> QSSVTLFGIVDTNVAYVNKDAAGDSRYGLGTSGASTSRLGLRGTEDLGGGLKAGFWLEGEIFGDDGNASGFNFKRRSTVSLSGNFGEVRLGRDLVPTSQKLTSYDLFSATGIGPFMGFRNWAAGQGADDNGIRANNLISYYTPNFGGFNAGFGYAFDEKQTIGTADSVGRYIGGYVAYDNGPLSASLGLAQQKTAVGGLATDRDEITLGASYN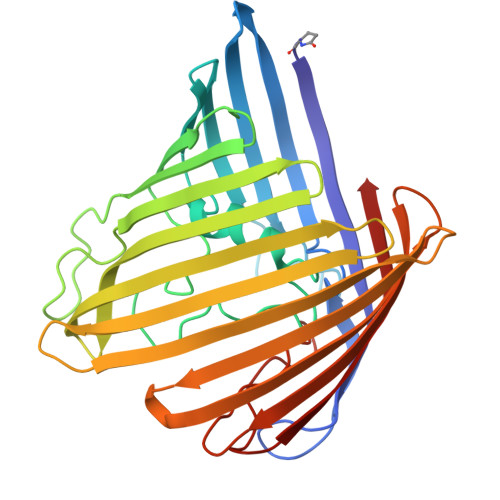FGVAKLSGLLQQTKFKRDIGGDIKTNSYMLGASAPVGGVGEVKLQYALYDQKAIDSKAHQITLGYVHNLSKRTALYGNLAFLKNKDASTLGLQAKGVYAGGVQAGESQTGVQVGIRHAF>MDQWSMLRHFDHITKDYHDHIAEISAKLVAIMDSLFDKLLSKYEVKAPVPSPCFRNICKQMTKMHEAIFDLLPEEQTQMLF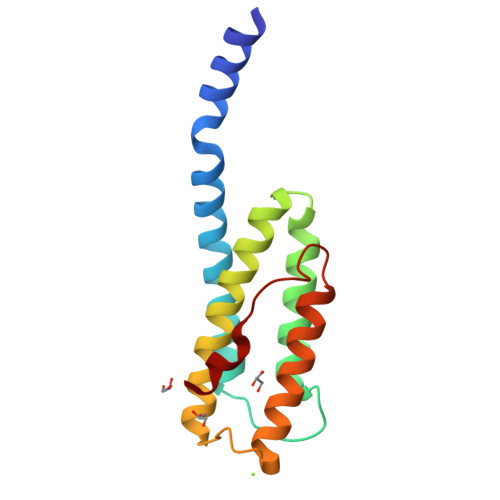LRINASYKLHLKKQLSHLNVINDGGPQNGLVTADVAFYTGNLQALKGLKDLDLNMAEIWE[2x]>[8x]GSHMASPSNTDYPGPHSFDVSFQQSSTAKSATWTYSTELKKLYCQIAKTCPIQIKVMTPPPQGAVI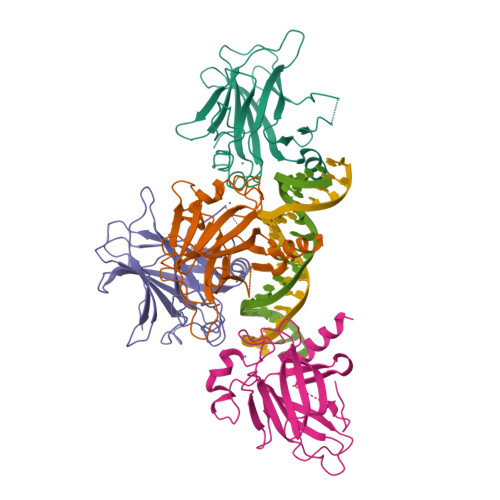RAMPVYKKAEHVTEVVKRCPNHELSREFNEGQIAPPSHLIRVEGNSHAQYVEDPITGRQSVLVPYEPPQVGTEFTTVLYNFMCNSSCVGGMNRRPILIIVTLETRDGQVLGRRCFEARICACPGRDRKADEDSIRKQ>[2x]GCTTAATT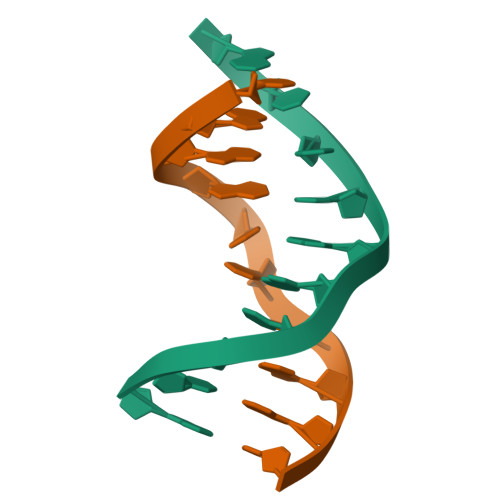CG;>[2x]CGAATTAAGC5-chloro-N-{[(4S)-4-(1-methyl-1H-imidazol-2-yl)-2,5-dioxoimidazolidin-4-yl]methyl}-1-benzofuran-2-carboxamide | C17 H14 Cl N5 O4 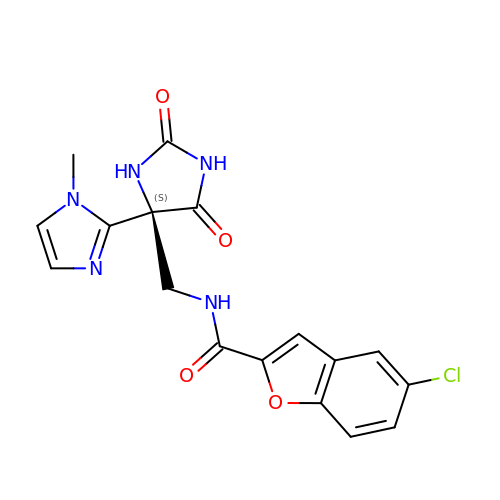| NPWGFJCNOCYDSO-KRWDZBQOSA-N>TAHRFLFVSTPVGPLGSGRGGGVELTLPNLAKALTQRGHQVSVLAPAGSVLPDLPLETVPGTWQSTAQSHGRATPAEIPAE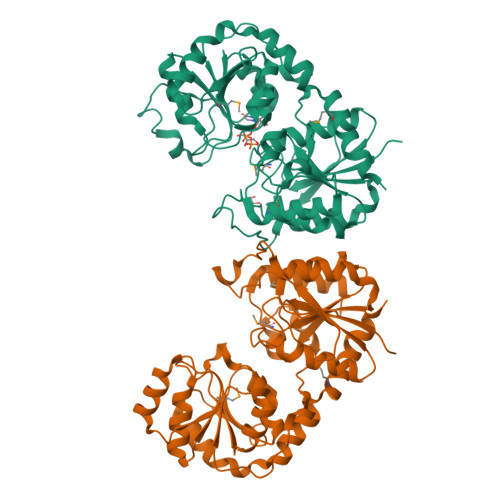SVLARLWDRAHQQQADFDLILNFAYDWLPLYLTPFFKTPVAHLISMGSLSEVMDQAIATSLDRYPGSIAVHSLAQAATFPFGDRCLCIGNALDLAAYGFNPEPEPVLGWVGRIAPEKGLEDAIQAAQQAGLPLRVWGALTEPDYWQRLQQQFGDRAVSYQGFVSTDELQRGLGRCQGLLMTPKWVEAFGNVAIEALACGLPVIAYARGGPLEIIEQGKSGWLVEPDQQAALVNAIGQLSSLDRAYCRAQAEARFSLAAMGQRLEAWLLPLLS[2x]>[4x]MRGSHHHHHHGMASHITYDLPVAIEDILEAKKRLAGKIYKTGMPRSNYFSERCKGEIFLKFENMQRTGSFKIRGAFNKLSSLTEAEKRKGVVACSAGNHAQGVSLSCAMLGIDGKVVMPKGAPKSKVAAT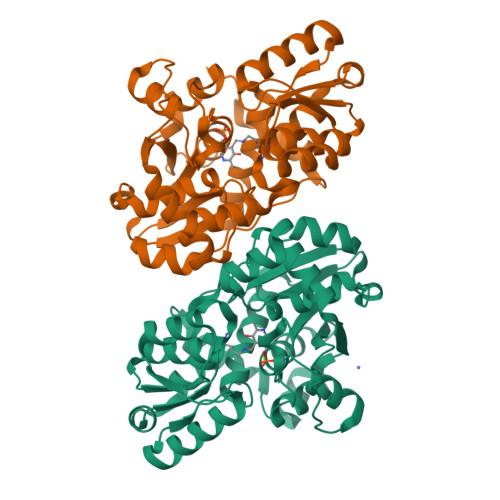CDYSAEVVLHGDNFNDTIAKVSEIVETEGRIFIPPYDDPKVIAGQGTIGLEIMEDLYDVDNVIVPIGGGGLIAGIAIAIKSINPTIKVIGVQAENVHGMAASYYTGEITTHRTTGTLADGCDVSRPGNLTYEIVRELVDDIVLVSEDEIRNSMIALIQRNKVITEGAGALACAALLSGKLDSHIQNRKTVSIISGGNIDLSRVSQITGLVDA>MASNFTQFVLVDNGGTGDVTVAPSNFANGVAEWISSNSRSQAYKVTCSVRQSSAQNRKYTIKVEVPKVATQTVGGVELPVAAWRSYLNMELTIPIFATNSDCELIVKAMQGLLKDGNPIPSAIAANSGIY[8x];> MRAFSTLDRENETFVPSVRVYADGETEDNSFSLKYRSNWTPGRFNSTGAKTKQWHYPSPYSRGALSVTSIDQGAYKRSGSSWGRPYEEKAGFGFSLDARSCYSLFPVSQNLTYIEVPQNVANRASTEVLQKVTQGNFNLGVALAEARSTASQLATQTIALVKAYTAARRGNWRQA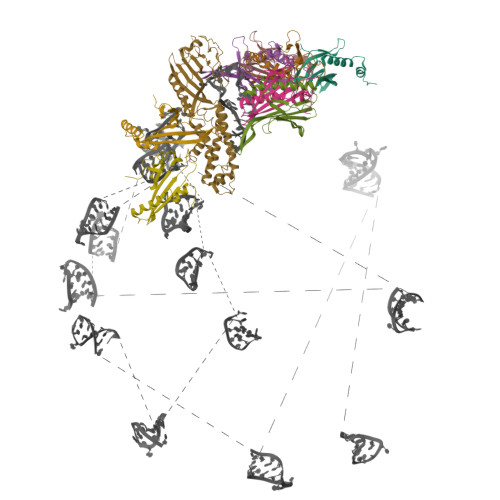LRYLALNEDRKFRSKHVAGRWLELQFGWLPLMSDIQGAYEMLTKVHLQEFLPMRAVRQVGTNIKLDGRLSYPAANFQTTCNISRRIVIWFYINDARLAWLSSLGILNPLGIVWEKVPFSFVVDWLLPVGNMLEGLTAPVGCSYMSGTVTDVITGESIISVDAPYGWTVERQGTAKAQISAMHRGVQSVWPTTGAYVKSPFSMVHTLDALALIRQRLSR> MEVCLPNGHQVVDLINNAFEGRVSIYSAQEGWDKTISAQPDMMVCGGAVVCMHCLGVVGSLQRKLKHLPHHRCNQQIRHQDYVDVQFADRVTAHWKRGMLSFVAQMHEMMNDVSPDDLDRVRTEGGSLVELNWLQVDPNSMFRSIHSSWTDPLQVVDDLDTKLDQYWTALNLMIDSSDLIPNFMMRDPSHAFNGVKLGGDARQTQFSRTFDSRSSLEWGVMVYDYSELEHDPSKGRAYRKELVTPARDFGHFGLSHYSRATTPILGKMPAVFSGMLTGNC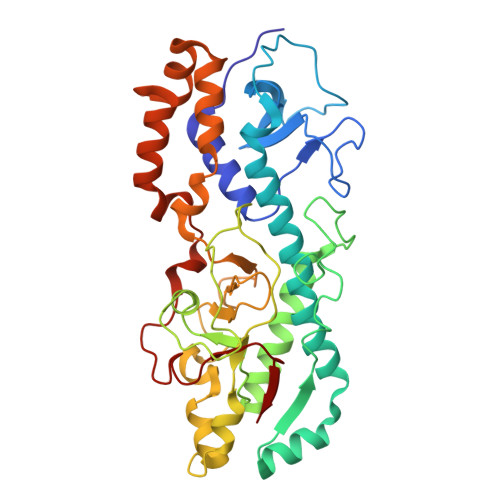KMYPFIKGTAKLKTVRKLVEAVNHAWGVEKIRYALGPGGMTGWYNRTMQQAPIVLTPAALTMFPDTIKFGDLNYPVMIGDPMILG> AEAGITGTWYAQLGSTFIVTAGADGALTGTYESAVGNAESRYVLTGRYDSAPATDGSGTALGWTVAWKNN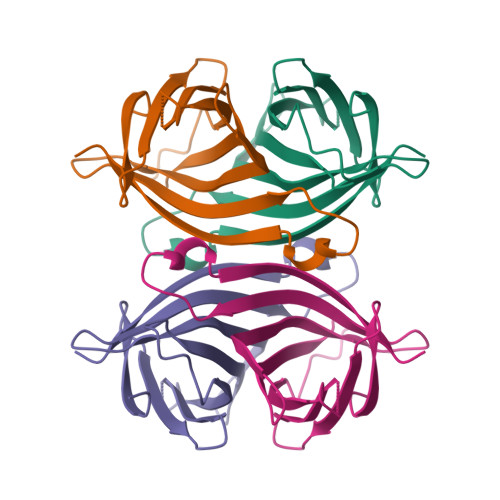YRNAHSATTWSGQYVGGAEARINTQWLLTSGTTEANAWKSTLVGHDTFTKVKPSAAS> GFPCGESCVYGPCFTAA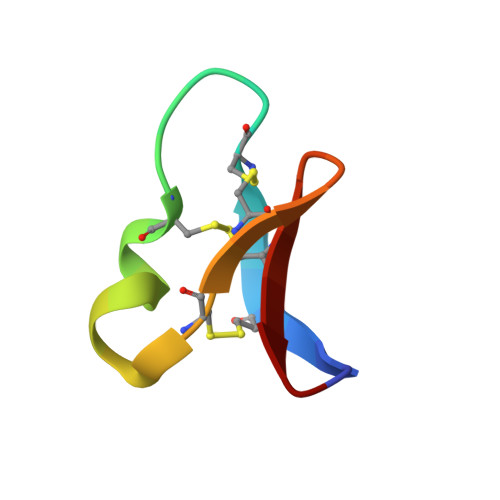IGCSCKSKVCYKN>MRGSHHHHHHGSMAVPPTYADLGKSARDVFTKGYGFGLIKLDLKTKSENGLEFTSSGSANTETTKVTGSLETKYRWTEYGLTFTEKWNTDNTLGTEITVEDQLARGLKLTFDSSFSPNTGKKNAKIKTGYKREHINLGCDMDFDIAGPSIRGALVLGYEGWLAGYQMNFETAKSRVTQSNFAVGYKTDEFQLHTNVND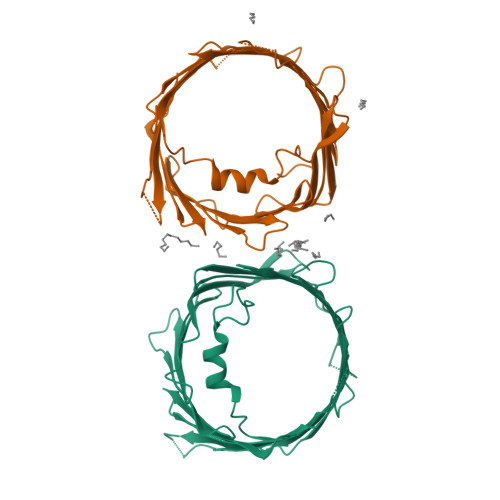GTEFGGSIYQKVNKKLETAVNLAWTAGNSNTRFGIAAKYQIDPDACFSAKVNNSSLIGLGYTQTLKPGIKLTLSALLDGKNVNAGGHKLGLGLEFQA[2x]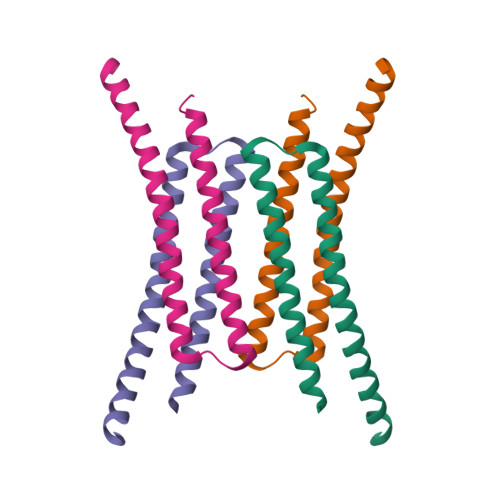>GSHMAPADYFRVLVQQFEVQLQQYRQQIEELENHLATQANNSHITPQDLSMAMQKIYQTFVALAAQLQSIHENVKVLKEQYLSYRKMFLGDAG[4x]> ADPAPVIEPSGPELVVEPGETVTLRCVSNGSVEWDGPISPYWTLDPESPGSTLTTRNATFKNTGTYRCTELEDPMAGSTTIHLYVKDPAHSWNLLAQEVTVVE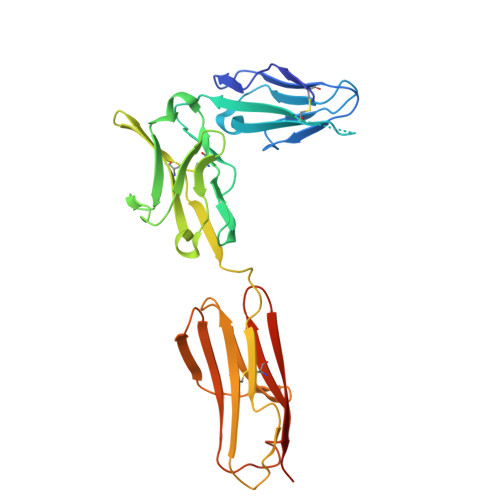GQEAVLPCLITDPALKDSVSLMREGGRQVLRKTVYFFSPWRGFIIRKAKVLDSNTYVCKTMVNGRESTSTGIWLKVNRVHPEPPQIKLEPSKLVRIRGEAAQIVCSATNAEVGFNVILKRGDTKLEIPLNSDFQDNYYKKVRALSLNAVDFQDAGIYSCVASNDVGTRTATMNFQVVESHHHHHHH> MTQAKAKHADVPVNLYRPNAPFIGKVISNEPLVKEGGIGIVQHIKFDLTGGNLKYIEGQSIGIIPPGVDKNGKPEKLRLYSIA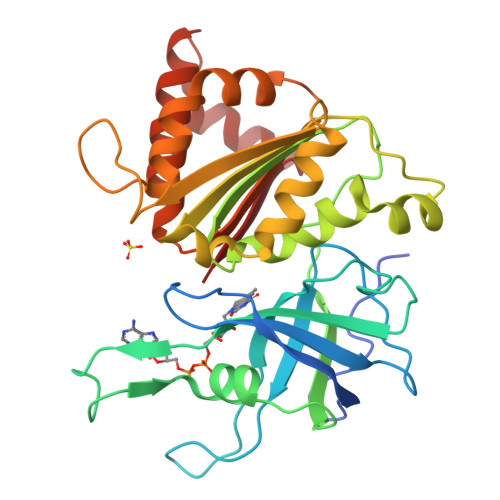STRHGDDVDDKTISLCVRQLEYKHPESGETVYGVCSTYLTHIEPGSEVKITGPVGKEMLLPDDPEANVIMLAGGTGITPMRTYLWRMFKDAERAANPEYQFKGFSWLVFGVPTTPNILYKEELEEIQQKYPDNFRLTYAISREQKNPQGGRMYIQDRVAEHADQLWQLIKNQKTHTYICGPPPMEEGIDAALSAAAAKEGVTWSDYQKDLKKAGRWHVETY> GAMGSKRQWALEDFEIGRPLGKGKFGNVYLAREKQSKFILALKVLFKAQ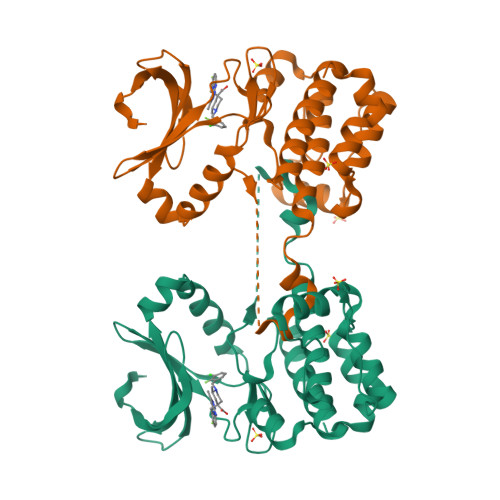LEKAGVEHQLRREVEIQSHLRHPNILRLYGYFHDATRVYLILEYAPLGTVYRELQKLSKFDEQRTATYITELANALSYCHSKRVIHRDIKPENLLLGSAGELKIADFGWSVHAPSSRRTTLCGTLDYLPPEMIEGRMHDEKVDLWSLGVLCYEFLVGKPPFEANTYQETYKRISRVEFTFPDFVTEGARDLISRLLKHNPSQRPMLREVLEHPWITANSSKPS> DCPSGWSSYEGNCYKFFQQKMNWADAERFCSEQAKGGHLVSIKI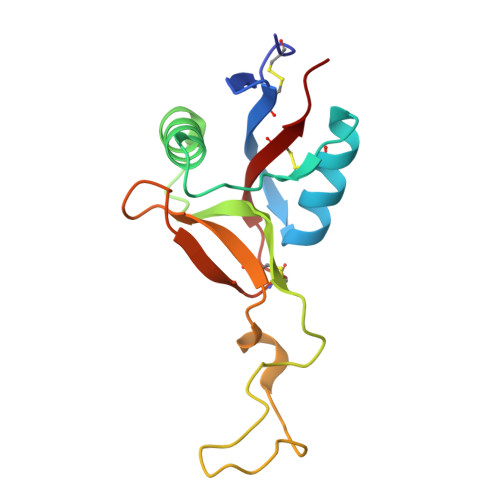YSKEKDFVGDLVTKNIQSSDLYAWIGLRVENKEKQCSSEWSDGSSVSYENVVERTVKKCFALEKDLGFVLWINLYCAQKNPFVCKSPPP>MISETIRSGDWKGEK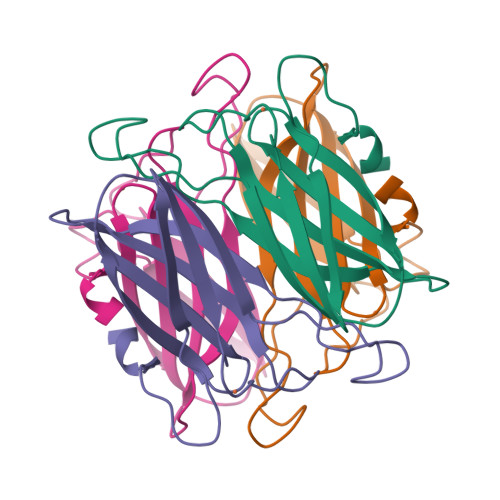HVPVIEYEREGELVKVKVQVGKEIPHPNTTEHHIRYIELYFLPEGENFVYQVGRVEFTAHGESVNGPNTSDVYTEPIAYFVLKTKKKGKLYALSYCNIHGLWENEVTLE[2x]> SNAGGSSPITGLVYDQRMMLHHNMWDSHHPELPQRISRIFSRHEELRLLSRCHRIPARLATEEELALCHSSKHISIIKSSEHMKPRDLNRLGDEYNSIFISNESYTCALLAAGSCFNSAQAILTGQV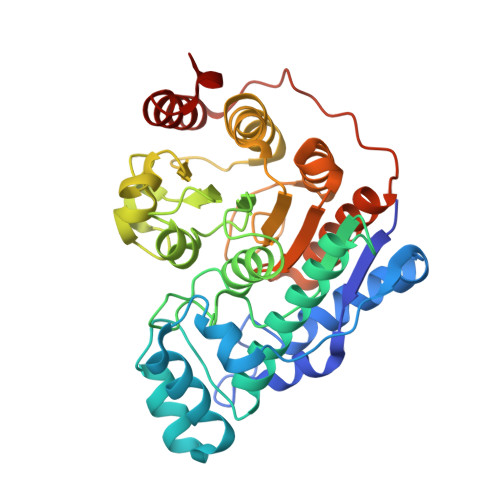RNAVAIVRPPGHAAEKDTACGFCFFNTAALTARYAQSITRESLRVLIVDWDVHHGNGTQHIFEEDDSVLYISLHRYEDGAFFPNSEDANYDKVGLGKGRGYNVNIPWNGGKMGDPEYMAAFHHLVMPIAREFAPELVLVSAGFDAARGDPLGGFQVTPEGYAHLTHQLMSLAAGRVLIILEGGYNLTSISESMSMCTSMLLGDSPPSLDHLTPLKTSATVSINNVLRAHAPFWSSLR> MTDGLNQLYNLVAQDY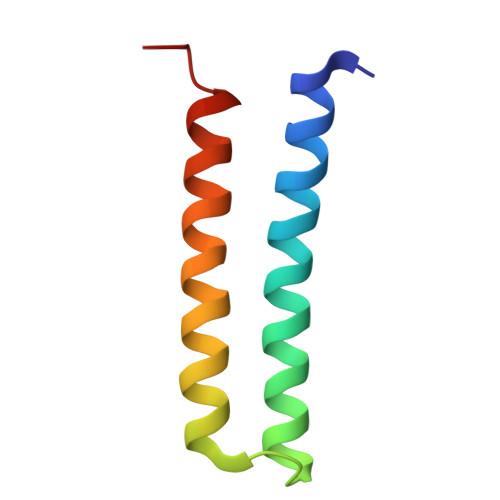ALTDTIEALSRMLHRGTIPLDTFVKQGRELARQQFLVRWHIQRITSPLS>MGGSHHHHHHGMASLAPGSSRVELFKRQSSKVPFEKDGKVTERVVHSFRLPALVNVDGVMVAIADARYETSFDNSLIDTVAKYSVDDGETWETQIAIKNSRASSVSRVVDPTVIVKGNKLYVLVGSYNSSRSYWTSHGDARDWDILLAVGEVTKSTAGGKITASIKWGSPVSLKEFFPAEMEGMHTNQFLGGAGVAIVASNGNLVYPVQVTNKKKQVFSKIFYSEDEGKTWKFGKGRSAFGCSEPVALEWEGKLIINTRVDYRRRLVYESSDMGNTWLEAVGTLSRVWGPSPKSNQPGSQSSFTAV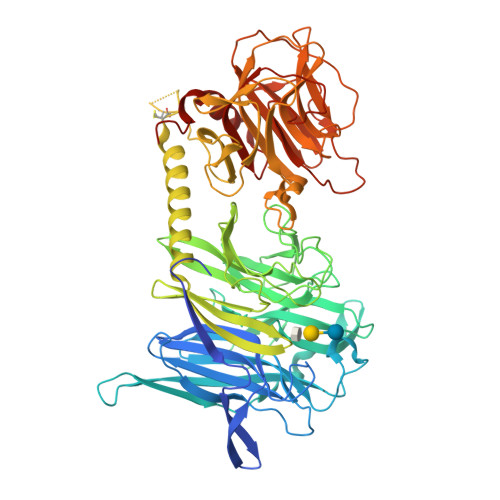TIEGMRVMLFTHPLNFKGRWLRDRLNLWLTDNQRIYNVGQVSIGDENSAYSSVLYKDDKLYCLHEINSNEVYSLVFARLVGELRIIKSVLQSWKNWDSHLSSICTPADPAASSSERGCGPAVTTVGLVGFLSHSATKTEWEDAYRCVNASTANAERVPNGLKFAGVGGGALWPVSQQGQNQRYHFANHAFTLVASVTIHEVPKGASPLLGASLDSSGGKKLLGLSYDKRHQWQPIYGSTPVTPTGSWEMGKRYHVVLTMANKIGSVYIDGEPLEGSGQTVVPDERTPDISHFYVGGYKRSGMPTDSRVTVNNVLLYNRQLNAEEIRTLFLSQDLIGTEAHMD[2x]>[2x]GAPATVTEQGEDITSKKDRGVLKIVKRVGNGEETPMIGDKVYVHYKGKLSNGKKFDSSHDRNEPFVFSLGKGQVIKAWDIGVATMKKGEIAHLLIKPEYAYGSAGSLPKIPSNATL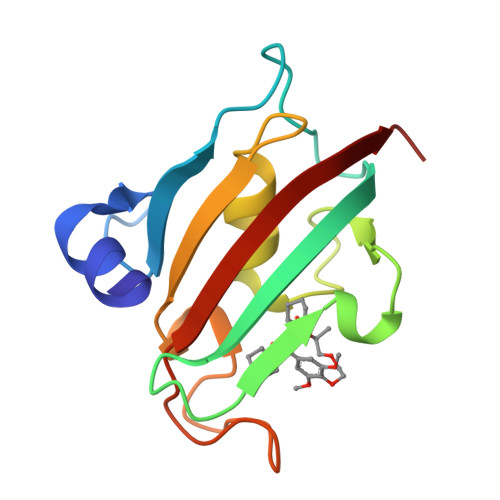FFEIELLDFKGE> MDLKKYKQKLIGSDEERAVSPVIGVILMVAITVILAAVIAAFVLDLGGSVGNEAQAGVNMEVDESQGGNITVEVTSMGNADHVVLGGSIDSDQTPYQGSSKNTGKLKLTVGDSVTINANNDGSVANYGLSSTE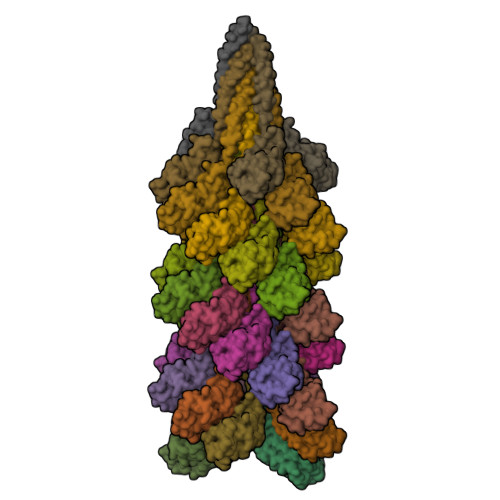GTVTAIAVIEEDETRTQVASVDYSGFTAKDIS>[2x]GPQMNYEEVIKKYRGEENFDHAAYDWRLHSGVTPVKDQKNCGSAWAFSSIGSVESQYAIRKNKLITLSEQELVDCSFKNYGCNGGLINNAFEDMIELGGICPDGDYPYVSDA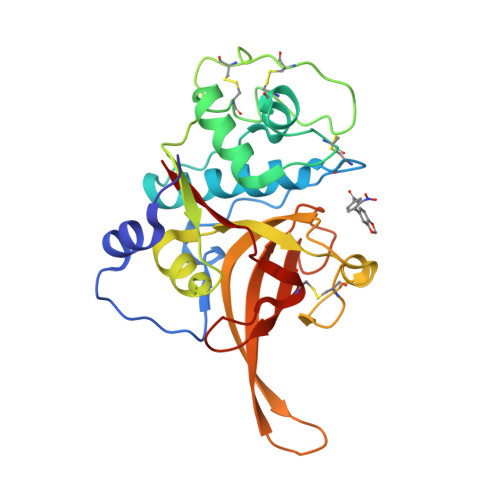PNLCNIDRCTEKYGIKNYLSVPDNKLKEALRFLGPISISVAVSDDFAFYKEGIFDGECGDQLNHAVMLVGFGMKEIVNPLTKKGEKHYYYIIKNSWGQQWGERGFINIETDESGLMRKCGLGTDAFIPLI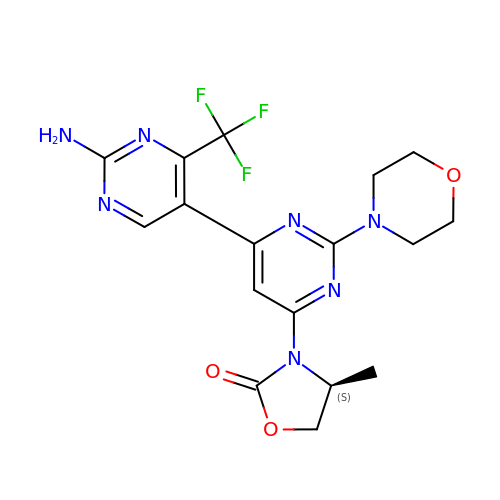(4~{S})-3-[6-[2-azanyl-4-(trifluoromethyl)pyrimidin-5-yl]-2-morpholin-4-yl-pyrimidin-4-yl]-4-methyl-1,3-oxazolidin-2-one | C17 H18 F3 N7 O3 | FBOZVYXXWXOUOV-VIFPVBQESA-N> MSLGAKPFGEKKFIEIKGRRMAYIDEGTGDPILFQHGNPTSSYLWRNIMPHCAGLGRLIACDLIGMGDSDKLDPSGPERYTYAEHRDYLDALWEALDLGDRVVLVVHDWGSALGFDWARRHRERVQGIAYMEAVTMPLEWADFPEQDRDLFQAFRSQAGEELVLQDNVFVEQVLPGLILRPLSEAEMAAYREPFLAAGEARRPTLSWPRQIPIAGTPADVVAIARDYAGWLSESPIPKLFINAEPGHLTTGRIRDFCRTWPNQTEITVAGAHFIQEDSPDEI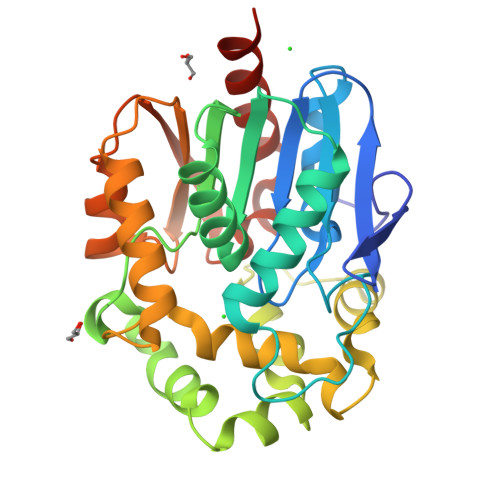GAAIAAFVRRLRPAHHHHHH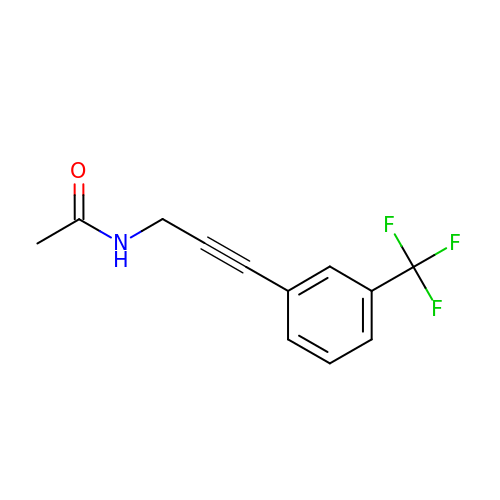N-{3-[3-(trifluoromethyl)phenyl]prop-2-yn-1-yl}acetamide | C12 H10 F3 N O | UYLIEUNFURJQLH-UHFFFAOYSA-N> 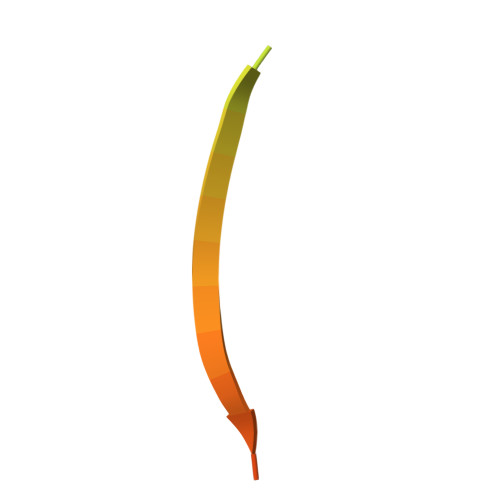YRRFEKEKLKSQWNNDNPLFKSATTTVMNPKFAES To combat these defenses, Anopheles mosquitoes produce inhibitors belonging to the SG7 protein family that block complement at the alternative C3 convertase, C3bBb. Crystal structures of albicin and SG7.AF reveal a novel four-helix bundle arrangement that is stabilized by an N-terminal hydrogen bonding network. In this study, we describe the structures of albicin and its orthologs SG7.AF (from An. freeborni) and anophensin (from An. stephensi), characterize the binding and mechanism of AP inhibition by these inhibitors, and determine a role for properdin in modulating the inhibitory activity of SG7.AF. SG7 family members are quite similar to one another structurally, but amino acid sequence divergence suggests that specific side chain interactions are key determinants for the observed differences in target affinity.

Here we show that SG7.AF, the albicin homolog from An. freeborni, has a similar potency to albicin but is more active in the presence of properdin, a plasma protein that acts to stabilize C3bBb. The backbone structure of SG7.AF is very similar to that of albicin (RMSD = 0.51 Å), with the lengths of the helices and positions of the cysteine residues being essentially the same. SG7.AF also contains an N-terminal structure identical to that of albicin where the amino group is stabilized by means of the same hydrogen bonding network. The IC50 value for SG7.AF was similar to that of albicin in NHS but increased by sixfold in PDS suggesting a role for properdin in its mechanism of action. Identically to albicin, SG7.AF showed no ability to inhibit the CP. The fact that SG7.AF remained inhibitory, albeit less so, in the absence of properdin indicates that it does not function simply as a scavenger of properdin, but rather is made more potent in its anti-C3bBb activity by properdin. Like albicin, SG7.AF did not block the activation of factor B by factor D (conversion of C3bB to C3bBb) demonstrating that it targets the C3bBb complex directly, rather than inhibiting the serine protease responsible for its activation. Together, these data suggest that SG7.AF acts similarly to albicin in that it inhibits the catalytic activity of the C3bBb complex by directly interacting with it. When injected along with C3b, factor B, and factor D, SG7.AF and albicin both cause an enhanced accumulation of C3bBb on the surface, but SG7.AF was required at higher concentrations, indicating a lower-affinity binding interaction for this inhibitor.

> ARKHVQELLKTFRRIDFDETRKSVYLQSAKFGVQSQLREPLTKKVLNYWDDVKLSKTCLDRMVTKVNDVKETFYAGFSYACESHNQYSVDCLEAAKPSYLTALGEIRGETEKCLTTRLK> MAHHHHHHVDDDDKGGLGEYGQRFMWLWNKIHDPANGYFNQDGIPYHSVETLICEAPDYGHLTTSEAFSYYVWLEAVYGKLTGDWSKFKTAWDTLEKYMIPSAEDQPMRSYDPNKPATYAGEWETPDKYPSPLEFNVPVGKDPLHNELVSTYGSTLMYGMHWLMDVDNWYGYGKRGDGVSRASFINTFQRGPEESVWETVPHPSWEEFKWGGPNGFLDLFIKDQNYSKQWRYTNAPDADARAIQATYWAKEWAKEQGKFNEISSYVAKAAKMGDYLRYAMFDKYFKPLGCQDKNAAGGTGYDSAHYLLSWYYAWGGALDGAWSWKIGCSHAHFGYQNPMAAWALANDSDMKPKSPNGASDWAKSLKRQIEFYRWLQSAEGAIAGGATNSWNGRYEKYPAGTATFYGMAYEPNPVYRDPGSNTWFGFQAW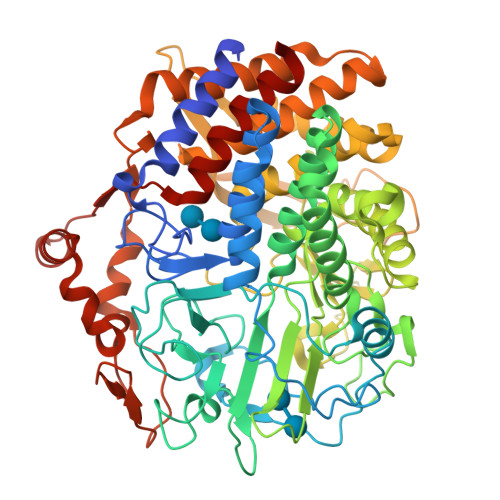SMQRVAEYYYVTGDKDAGALLEKWVSWIKSVVKLNSDGTFAIPSTLDWSGQPDTWNGTYTGNPNLHVKVVDYGTDLGITASLANALLYYSAATKKYGVFDEEAKNLAKELLDRMWKLYRDEKGLSAPEKRADYKRFFEQEVYIPAGWTGKMPNGDVIKSGVKFIDIRSKYKQDPDWPKLEAAYKSGQVPEFRYHRFWAQCDIAIANATYEILFGNQ> AQSVPYGVSQIKAPALHSQGYTGSNVKVAVIDSGIDSSHPDLKVAGGASMVPSETNPFQDNNSHGTHVAGTVAALNNSIGVLGVAPSASLYAVKVLGADGSGQYSWIINGIEWAIANNMDVINMSLGGPSGSAALKAAVDKAVASGVVVVAAAGNEGTSGSSSTVGYPGKYPSVIAVGAVDSSNQRASFS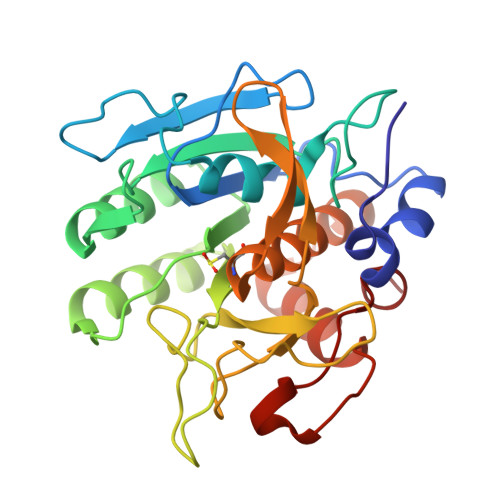SVGPELDVMAPGVSIQSTLPGNKYGAYNGTCMASPHVAGAAALILSKHPNWTNTQVRSSLENTTTKLGDSFYYGKGLINVQAAAQ> PQDADKLPHTKVTLVAPPQVHPHEQATKSGPKVVEFTMTIEEKKMVIDDKGTTLQAMTFNGSMPGPTLVVHEGDYVQLTLVN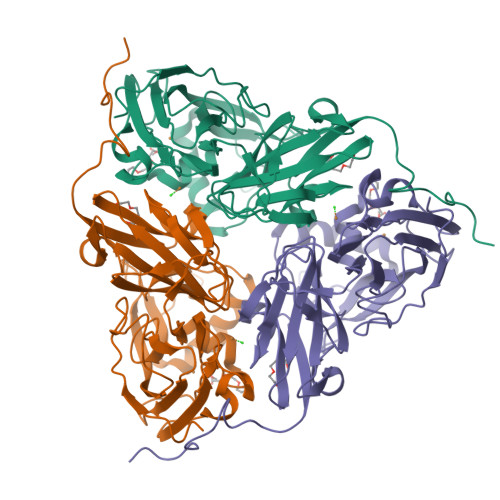PATNAMPHNVDFHGATGALGGAKLTNVNPGEQATLRFKADRSGTFVYHCAPEGMVPWHVVSGMSGTLMVLPRDGLKDPQGKPLHYDRAYTIGEFDLYIPKGPDGKYKDYATLAESYGDTVQVMRTLTPSHIVFNGKVGALTGANALTAKVGETVLLIHSQANRDTRPHLIGGHGDWVWETGKFANPPQRDLETWFIRGGSAGAALYTFKQPGVYAYLNHNLIEAFELGAAGHIKVEGKWNDDLMKQIKAPAPIPR> MGSLKGDHNIRVAILDGPVDIAHPCFQGADLTVLPTLAPTAARSDGFMSAHGTHVASIIFGQPETSVPGIAPQCRGLIVPIFSDDRRRITQLDLARGIERA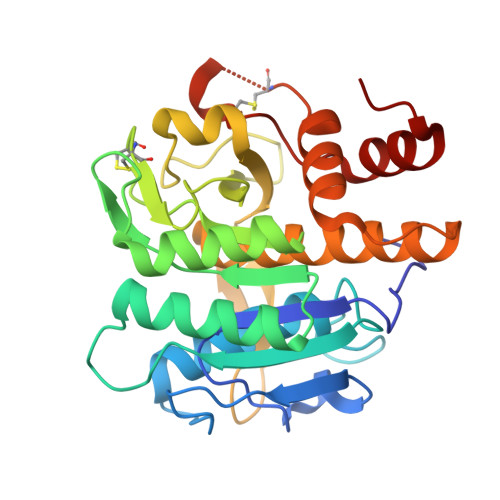VNAGAHIINISGGELTDFGEADGWLENAVSLCRQNNVLLVAAAGNNGCDCLHVPAALPAVLAVGAMDDHGHPLDFSNWGSTYEQQGILAPGEDILGAKPGGGTERLSGTAFATPIVSGVAALLLSEQVRRGETPDPQKVRQLLLQSALPCDDDAPEQARRCLAGRLNVSGAFTLLKGGDMS>[2x]QEGLDFPEYDGVDRVINVNAKNYKNVFKKYEVLALLYHEPPEDDKASQRQFETE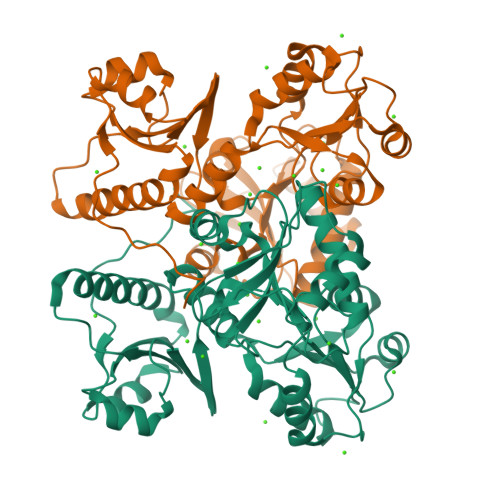ELILELAAQVLEDKGVGFGLVDSEKDAAVAKKLGLTEVDSMYVFKGDEVIEYDGEFSADTIVEFLLDVLEDPVELIEGERELQAFENIEDEIKLIGYFKSKDSEHYKAFEDAAEEFHPYIPFFATFDSKVAKKLTLKLNEIDFYEAFMEEPVTIPDKPNSEEEIVNFVEEHRRSTLRKLKPESMYETWEDDMDGIHIVAFAEEADPDGFEFLETLKAVAQDNTENPDLSIIWIDPDDFPLLVPYWEKTFDIDLSAPQIGVVNVTDADSVWMEMDDEEDLPSAEELEDWLEDVLEGEINTEDDDDDDDD> AKVEVGDEVGNFKFYPDSITVSAGEAVEFTLVGETPHNIVFDIPAGAPGTVASELKAASMDENDLLSED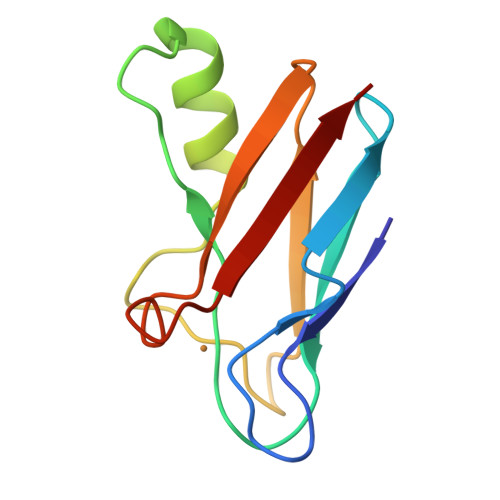EPSFKAKVSTPGTYTFYCTPHKSANMKGTLTVK> MELDDFDPEDKEILSWDINDVKLPQNVKTTDWFQEWPDSYVKHIYSSDDRNAQRHLSSWAMRNTNNHNSRILKKSCLGVVVCSRDCSTEEGRKIYLRPAICDKARQKQQRKSCPNCNGPLKLIPC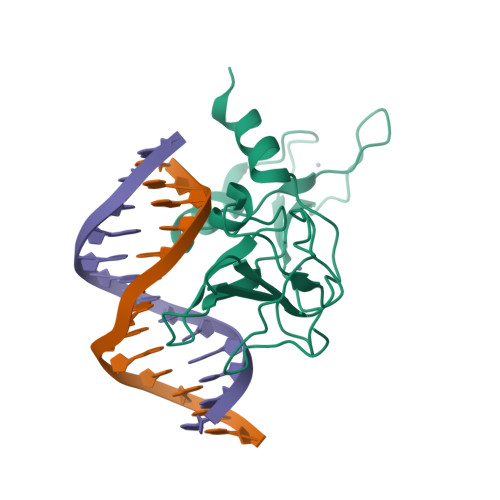RGHGGFPVTNFWRHDGRFIFFQSKGEHDHPRPETKLEAEARRAMKKVHM>MTTVQLTDVQTLRDRARKNIQEGAVTEGYSADRQTVLRLLNEALATELVCFLRYKRHYFMATGLKASIAAAEFLEHANQEMQHADQLAERIMQLGGEPDFNPRGLEERSHAEYVEGKTLKDMVTENLIAERIAIDSYREIITYLGNDDPTTRRIFEEILAQEEEHADDMADILDDLA[12x]

We report the biochemical, structural, and functional characterization of the protein coded by gene PA4880 in the P. aeruginosa PAO1 genome. Our structural work shows that the product of gene PA4880 is a protein that adopts the Dps subunit fold, which oligomerizes into a 12-mer quaternary structure. Unlike Dps, however, the ferroxidase di-iron centers and iron coordinating ligands are buried within each subunit, in a manner identical to that observed in the ferroxidase center of P. aeruginosa bacterioferritin. The ferroxidase centers in Pa DpsL catalyze the oxidation of Fe2+ utilizing O2 or H2O2 as oxidant, and the resultant Fe3+ is compartmentalized in the interior cavity.

Protein purification in the presence of MgSO4 enabled isolation of dodecameric DpsL in high yield. The protein was used to screen crystallization conditions leading to the formation of prismatic crystals from the Salt Rx HT screen condition F9 (800 mM lithium sulfate, 100 mM Tris pH 8.5). X-ray diffraction from these crystals, followed by structure solution and refinement produced the model termed Pa DpsL-dd (2.9 Å resolution), which contains 12 molecules (a dodecamer) in the asymmetric unit, 33 sulfate ions and 24 Fe ions. The sulfate ions are in the 3-fold pores and near sites containing R13, R33, and R103. Each of the subunits exhibit a Dps fold identical to that depicted in Figure 2A, except that the position of N-terminal residues D8–S30 is made evident in the 12-mer structure by well-defined electron density. Consequently, the structure of the dodecamer corroborated that each of the subunits in Pa DpsL exhibit a characteristic Dps fold that harbors a ferroxidase center typical of bacterioferritin. Sulfate site 1 is located next to each N-terminal extension, where the electrostatic interactions between SO4 2- and the side chains of Arg13 and Arg17 stabilize the two-turn helix observed in the N-terminal extension. As is typical of the Dps quaternary structure, each of the two three-fold pores along a three-fold axis has a different microenvironment, thus resulting in two types of three-fold pores, termed here A and B. Each of the type-A three-fold pores, which are formed by residues near the turn separating α1 and α2 contain a SO4 2- (site 3), which interacts electrostatically with the three Lys65 residues at the pore.>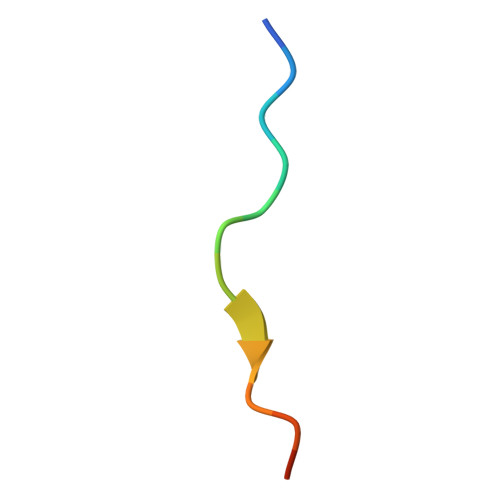 EVRQKKRRKRSTSR>[5x]MSEFRIHHDVNELLSLLRVHGGDGAEVYIDLLQKNRTPYVTTTVSAHSAKVKIAEFSRTPEDFLKKYDELKSKNTRNLDPLVYLLSKLMEDRETLQYLQQNAKERAELAASAAASSTASFGASATASKISMQELEELRKQLGSVATGPTWQQSLELTRKMLRDKQSKKNSGQRLPVLPAWVYERPALLGDFLPGTGGSADTAVPIGSLPLASQEAAVVEDLLYVLVGVDGRYISAQPLTGRQGRTFLVDPNLDLSIRELVSRILPVAASYSTVTRFIEEKSSFEYGQVNHALAAAMRTLVKEYLVLVTQLEQLQRQGLLSLQKLWFYIQPAMRSLDILASLATSVDKGECIGGATLSLLHDRSFSYTGDSQAQELCLHLTKAASTPYFEILEKWIYRGIIDDPYSEFMVEEHELRKEKIQEDYNDKYWDQRYTVVQRQIPSFLQKMAGKVLSTGKYLNVVRECGHDVTCPVAKEVVYTLKERAYVEQIEKAFSYASKVLLDFLMGEKELLAHLRSIKRYFLMDQGDFFVHFMDLTEEELKKPVDDITPTRLEALLELALRMSTANTDPFKDDLKIDLMPHDLITQLLRVLAIETQQEKAMVHADPTELTLSGLEAFSFDYVVTWPLSLIINRKALTRYQMLFRHMFYCKHVERQLCSVWISNKAAKRFSLHSAKWFAGAFTLRQRMLNFVQNIQSYMMFEVMEPTWHVLEQNLRSASNIDDVLGHHASFLDNCLKDCMLTNPELLRVFSKLMSVCVMFTNCLQRFTQSMKLDSELGHPALEPGAMLGPPTEAERAEERARKELARKCLAEHVDAPQLASSFEATITKFDKNFSAHLLDLLARLSIYSTSDCEHGMASVISRLDFNGFYTERLERLSAERSQKAAPPVPGPRGPPALVPRVAVTAQ;>MATPDQKSPNVLLQNLCCRILGKSEADVAQQFQYAVRVIGSNFAPTVERDEFLVAEKIKKELTRQRREADAALFSELHRKLHSQGVLKNKWSILYLLLSLSEDPRKQPSKVSGYAALFAQALPRDAHSTPYYYARPQSLPLNYQERGAPSAQSAGSAGSSGVSSLGTYALNGPTPPPPPPALLPGQPLPAPGVGDGLRQQLGSRLAWTLTASQPSLPSTTSKAVPSSGSRGAARPRREGDAAAGAVEVTEAALVRDILYVFQGIDGKHVKMSNADNCYTVEGKANLSKSLRDTAVRLAELGWLHNKIRKYTDQRSLDRSFGLVGQSFCAALHQELREYYRLLSVLHSQLQLEDDQGVNLGLESSLTLRRLLVWTYDPKMRLKTLAALVDHCQGRKGGELASAVHAYTKTGDPYARSLVQHILSLVSHPVLSFLYRWIYDGELEDTYHEFFVASDPAVKADRLWHDKYALRKPMIPSFMTMDQCRKVLLIGKSINFLHQVCHDQTPTTKMIAVTKSAESPQDAADLFTDLENAFQGKIDAAYFETSKYLLDVLNKKYSLLDHMQAMRRYLLLGQGDFIRHLMDLLKPELVRPATTLYQHNLTGILETAVRATNAQFDSPEILKRLDVRLLEVSPGDTGWDVFSLDYHVDGPIATVFTRECMSHYLRAFNFLWRAKRVEYILTDIRKGHMCNARLLRSMPEFSGVLHHCHILASEMVHFIHQMQYYVTFEVLECSWDELWNRVQRAQDLDHIIAAHEAFLGTVISRCLLDSDSRALLNQLRAVFDQIIELQNTQDAIYRAALEELQRRLQFEEKKKQREAEGQWGVSAAEEEQEKRRVQEFQESIPKMCSQLRILTHFYQGVVQQFLVSLTTSSDESLRFLSFRLDFNEHYRAREPRLRVSLGTRGRRSSHT[5x];>MIHELLLALSGYPGSIFTWNKRGGLQVSQDFPFLHPSETSVLNRLCRLGTDYIRFTEFIEQYTGHVQQQDHHPSQQGQGGLHGIYLRAFCTGLDSVLQPYRQALLDLEQEFLADPHLSISHINYSLDQFQLLFPSVMVVVEQIKSQKIHGCQILETVYKHSCGGLPPVRSALEKILAVCHGVMYKQLSAWMLHGLLLDQHEEFFIKQGPSSGNVSAQPEEDEEDLGIGGLTGKQLRELQDLRLIEEENMLAPSLKQFSLRVEILPSYIPVRVAEKILFVGESVQMFENQNVNLTRKGSILKDQEDTFAAELHRLKQQPLFSLVDFEQVVDRIRSTVAEHLWKLMVEESDLLGQLKIIKDFYLLGRGELFQAFIDTAQHMLKTPPTAVTEHDVNVAFQQSAHKVLLDDDNLLPLLHLTIEYHGKEHKADATQAREGPSRETSPREAPASGWAALGLSYKVQWPLHILFTPAVLEKYNVVFKYLLSVRRVQAELQHCWALQMQRKHLKSNQTDAVKWRLRNHMAFLVDNLQYYLQVDVLESQFSQLLHQINSTRDFESIRLAHDHFLSNLLAQSFILLKPVFHCLNEILDLCHSFCSLVSQNLGPLDERGAAQLSILVKGFSRQSSLLFKILSSVRNHQINSDLAQLLLRLDYNKYYTQAGGTLGSFGM[2x];> MASPAPSWTRLDPQQERDVRELIRLVSGVQDEADPNFQLALHFAWSNFRFHRFLDVNSHKVEKTIEGIYEKFIIHSDLSKAASWKRLTDEFLNASLPSIKEIKTDAHYSILSLLLCLSDSPSNSNYVETPRNKEVEKKDDFDWGKYLMEGEEIDLGPNVDTPNWSEESEDEDDPQPLSREDSGIQVDRTPLEEQDQSRKPASRVSWKVDEPDARSWLEQHVVRQYWTTRSSKFPHSLHLHSNLAAVWDQHLYSSDPLYVPDDRVSVTETQVIRETLWLLSGVKKLFIFQLIDGKVAVRNNIMVTHLTHSCLRSVLEQIAAYGQVVFRLQEFIDEVMGHSSESTLPGNGSVPKKSTDAPFRTYQAFMWALYKYFISFKEELSEIEKCIINNDTTVTLAIVVDKLSPRLAQLKVLHKVFSTGVAEVPPDTRNVVRASHLLNTLYKAILEYDNVGEASEQTVSLLFSLWVETVRPYLQIVDEWIVHGHLCDGAREFIIQRNKNVPVNHRDFWYATYTLYSVSEKTENEEKMSDNASASSGSDQGPSSRQHTMVSFLKPVLKQIIMAGKSMQLLKNLQCAESTTCQAMARDAERKSLYTLFLESVQSRLRHGEDATAQALTEQQATRETLIKMQSIAERHLELDDVHDPLLAINFARLYLEQSDFHEKFAGGDICVDRSSESVTCQTFELTLRSCLYPHIDKQYLDCCGNLMRTLKKDYRLVEYLQAMRNFFLMEGGDTMYDFYTSIFDKIREKETWQNVSFLNVQLQEAVGQRYPEDSSRLSISFENTDTAKKKLPVHTLDGLTLSYKVPWPVDIVISLECQKIYNQVFLLLLQIKWAKYSLDVLLFGELASSAEKPQSKEGLLSGQDTAAQFGPQKEPVRQQIHRMFLLRVKLMHFVNSLHNYIMTRILHSTGLEFQHQVEEAKDLDQLIKIHYRYLSTIHDRCLLREKVSFVKEAIMKVLNLALMFADGWQAGLGAWQMESIEKMESDFKNCHMFLVTILNKAVCRGSFPHLESLALSLMAGMEQKREDDLFNHTWGQGDLPNYTCAVRLLGVRKGGGTRPK;> MASVPQLLDDLCEALLPAAKAHLGQRRGSRKRAKQSLKKVAYNALFTNLFQDEARKLQPDLPRLPVKNRILMLSFDLRVGGLAAEADRLEELVEGLETAPRGPLAELGSVLDLLVQLAGSGPPRVLQRRRDYFLPKEHVGRNVRYGGYDCCHLSGIEADVRSIISGEEELCRDLIRKTLQVMEAAPGTGLPAFGLSSYGDPYGDRFERDTRVSLFGALVHSRTADLDVRLDLPPVPDSADVSGLAIKVPLSVDQSEDEGFQSAPNLTPDSQSEPGVTPDIDLWEAVLTYEASRRRCWEQIGCPPGHREEPYLTEAGRDAFDRFCRLRQGELQVLGGALLQAPQPVLVKESELVKDTLNVLLGVVSATFSLCQPAQAFTVKRGVHVSGASPESVSSLLSEVAECGTHYARLSDFSLQPVLDSSCSKGLVFQAFTSGLRRYLQYYRACVLSTPPTLSLLTIGFLFKKLGRQLRYLAELCGVGTALPGTGGG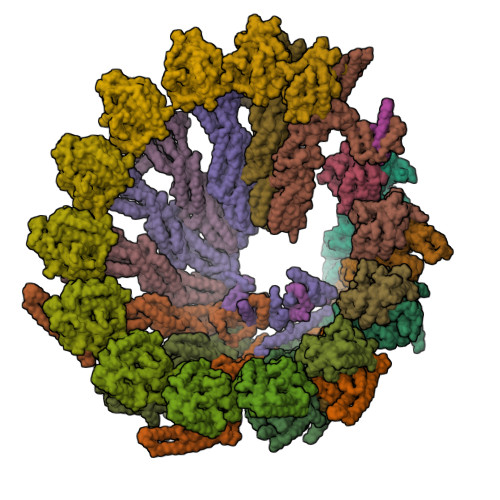EPRAAFPTGVRLLSYLYQEALDNCSNEHYPVLLSLLKTSCEPYTRFIHDWVYSGVFRDVYGEFMIQVNHEYLGCRDKSYWTHGYVLVSKEVEACVPVFLKHVAHDVYVCGKTINLLKLCCPRHYLCCSDVPVPRISVIFSLEELKDIEKDCAIYVGRMERVARHSSLSKEEKELRMEIAKQELIVHAREAASRVLSALSDRQMSERMALDARKREQFQRLKEQFMRDQERRRAARQEELDDDFSYARELRDRERRLKALEEQLERKARQALVDHYSKLSAEAARRERKALWRVQRHRLADARRRFLLEEEKRVQVMPSCSWERNQGALVFQASLPCPEHPDGGGGCGSGPSEQPKAARDGPRGPSRLMPQLPESPAEAACGLLSVGLSIRDFLPTAQGAEQPLHTGSALVLEEALQTIGSDLPPPAPSAAVGTGPSGPQEYDFRTILRPAVATSAFPGPLQSTGGGLGSEGQPQWEDTHVQLDMCVLDGQVALPHACSPQKTSPQEGSQAMGQLLRQVSEGDVPTGGYASGTAPSRPRWNVHGHVSDASIKVGENVCDVVPSRPRWNVHGHVSDASIKVGENVCDVVPSRPRWNVHGHVSDASIKVGENVCDVVPSRPRWNIHGHVSDASIKVGENVCDVVPSRPRWNVHGHVSQSQVTLGVLSGEAEPIVPWPHQTPPDHGSQSGLSLGAQSPAQEGEPQPAAETAVEGAESGPQASPTAGAGSSLLSGSRLGPEARPPPPPPHLFCPGRSEDTVDLPASCRPSSQVRGQGLGVGGESSAGCPSHPACPFMGNEGSVPGPGVDTQSSPGLGEEAAQRWGMEQAYLAGLAGQYRLEQYPDSYEAMSEPPVARLLHHGLPRAFALPEDSGVQPDTDETAVQLSELLPLPVLMKHSVTAPLAAHVSLVNKAAVDYFFVELHLGAHFEALRHFLLMEDGEFAQSLSDLLFEKLGAGQTPGELLSPLVLNSVLSKALQYSLHGDTPHAANLSFALKFLPEAFAPNAPDVLSCLELRYKVDWPLNIVVTEGCLSRYSGIFSFLLQLKLMMWTLKDVCFHLKRTARMSHVASSVQFRQLQLFKHEMQHFVKVIQGYIANQILHVTWCEFRARLASVGDLEEIQRAHAEYLHKAVFRGLLTEKAAPAMNIIHSLFSLVLKFRSQLISQPWGLAGGPHGAEHPNFALMQQSYSTFKYYSHFLFKVVSKLVNRGYQPHLEDFLLRINFNNYYQDA;>MAGNSGSGAAAAANLNAVRETMDVLLEISRILNTGLDMETLSICVRLCEQGINPEALSSVIKELRKATEALKAAENMTS[3x];>[4x]MAAPGAGPGPGAPPGLEAALQKLALRRKKVLSAEETELFELAQAAGGAMDPEVFKILVDLLKLNVAPLAVFQMLKSMCAGQRLASEPQDPVAVPLPTTSVPETRGRNRGSSALGGGPALAERSGREGSSQRMPRQPSATRLPKGGGPGKSPTRST;>[14x]MPREIITLQLGQCGNQIGFEFWKQLCAEHGISPEGIVEEFATEGTDRKDVFFYQADDEHYIPRAVLLDLEPRVIHSILNSPYAKLYNPENIYLSEHGGGAGNNWASGFSQGEKIHEDIFDIIDREADGSDSLEGFVLCHSIAGGTGSGLGSYLLERLNDRYPKKLVQTYSVFPNQDEMSDVVVQPYNSLLTLKRLTQNADCVVVLDNTALNRIATDRLHIQNPSFSQINQLVSTIMSASTTTLRYPGYMNNDLIGLIASLIPTPRLHFLMTGYTPLTTDQSVASVRKTTVLDVMRRLLQPKNVMVSTGRDRQTNHCYIAILNIIQGEVDPTQVHKSLQRIRERKLANFIPWGPASIQVALSRKSPYLPSAHRVSGLMMANHTSISSLFESSCQQYDKLRKREAFLEQFRKEDIFKENFDELDRSREVVQELIDEYHAATRPDYISWGTQEQ;>[10x]MMDLVLEEDVTVPGTLSGCSGLVPSVPDDLDGINPNAGLGNGLLPNVSEETVSPTRARNMKDFENQITELKKENFNLKLRIYFLEERMQQEFHGPTEHIYKTNIELKVEVESLKRELQEREQLLIKASKAVESLAEAGGSEIQRVKEDARKKVQQVEDLLTKRILLLEKDVTAAQAELEKAFAGTETEKALRLRLESKLSEMKKMHEGDLAMALVLDEKDRLIEELKLSLKSKEALIQCLKEEKSQMACPDENVSSGELRGLCAAPREEKERETEAAQMEHQKERNSFEERIQALEEDLREKEREIATEKKNSLKRDKAIQGLTMALKSKEKKVEELNSEIEKLSAAFAKAREALQKAQTQEFQGSEDYETALSGKEALSAALRSQNLTKSTENHRLRRSIKKITQELSDLQQERERLEKDLEEAHREKSKGDCTIRDLRNEVEKLRNEVNEREKAMENRYKSLLSESNKKLHNQEQVIKHLTESTNQKDVLLQKFNEKDLEVIQQNCYLMAAEDLELRSEGLITEKCSSQQPPGSKTIFSKEKKQSSDYEELIQVLKKEQDIYTHLVKSLQESDSINNLQAELNKIFALRKQLEQDVLSYQNLRKTLEEQISEIRRREESFSLYSDQTSYLSICLEENNRFQVEHFSQEELKKKVSDLIQLVKELYTDNQHLKKTIFDLSCMGFQGNGFPDRLASTEQTEEAKKSRLPILIKPSRSLGNMYRLPATQEVVTQLQSQILELQGELKEFKTCNKQLHQKLILAEAVMEGRPTPDKTLLNAQPPVGAAYQDSPGEQKGIKTTSSVWRDKEMDSDQQRSYEIDSEICPPDDLASLPSCKENPEDVLSPTSVATYLSSKSQPSAKVSVMGTDQSESINTSNETEYLKQKIHDLETELEGYQNFIFQLQKHSQCSEAIITVLCGTEGAQDGLSKPKNGSDGEEMTFSSLHQVRYVKHVKILGPLAPEMIDSRVLENLKQQLEEQEYKLQKEQNLNMQLFSEIHNLQNKFRDLSPPRYDSLVQSQARELSLQRQQIKDGHGICVISRQHMNTMIKAFEELLQASDVDYCVAEGFQEQLNQCAELLEKLEKLFLNGKSVGVEMNTQNELMERIEEDNLTYQHLLPESPEPSASHALSDYETSEKSFFSRDQKQDNETEKTSVMVNSFSQDLLMEHIQEIRTLRKRLEESIKTNEKLRKQLERQGSEFVQGSTSIFASGSELHSSLTSEIHFLRKQNQALNAMLIKGSRDKQKENDKLRESLSRKTVSLEHLQREYASVKEENERLQKEGSEKERHNQQLIQEVRCSGQELSRVQEEVKLRQQLLSQNDKLLQSLRVELKAYEKLDEEHRRLREASGEGWKGQDPFRDLHSLLMEIQALRLQLERSIETSSTLQSRLKEQLARGAEKAQEGALTLAVQAVSIPEVPLQPDKHDGDKYPMESDNSFDLFDSSQAVTPKSVSETPPLSGNDTDSLSCDSGSSATSTPCVSRLVTGHHLWASKNGRHVLGLIEDYEALLKQISQGQRLLAEMDIQTQEAPSSTSQELGTKGPHPAPLSKFVSSVSTAKLTLEEAYRRLKLLWRVSLPEDGQCPLHCEQIGEMKAEVTKLHKKLFEQEKKLQNTMKLLQLSKRQEKVIFDQLVVTHKILRKARGNLELRPGGAHPGTCSPSRPGS> MGDTKEQRILNHVLQHAEPGNAQSVLEAIDTYCEQ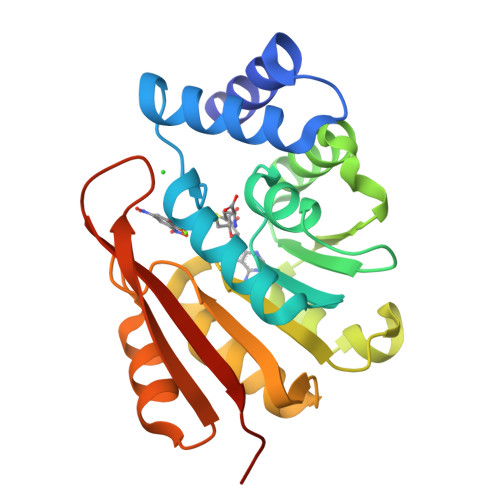KEWAMNVGDKKGKIVDAVIQEHQPSVLLELGAYCGYSAVRMARLLSPGARLITIEINPDCAAITQRMVDFAGVKDKVTLVVGASQDIIPQLKKKYDVDTLDMVFLDHWKDRYLPDTLLLEECGLLRKGTVLLADNVICPGAPDFLAHVRGSSCFECTHYQSFLEYREVVDGLEKAIYKGPGSEAGP> MTSTAVEITVKNAADIAIIGGSGLYQMQALTNKRSVKIETPYGEPSDDIVLGELNGVTVAFLTRHGQGHRLTPSEVPYRANIYALKTLGVRYIVSVSAVGSLQETLKPLDMVIPDQMIDMTKQRVSTFFGDGAVAHVSMADPLCPEVADILIRAYDNADIADGQCHAKATYVCIEGPQFSTRAESHWYRQMQADIIGMTNMPEAKLAREASIAYATLALVTDFDCWHPNEQAVSADYAIQNLMKNADNAQQVIKQAVALIASEQPKSIAHTALTQALVTPVEAMSAETKTRLAALLP

The monomer of RSFP has a mixed α-β architecture. The main structural motif is an eight stranded mixed β-sheet located in the centre of the monomer. On the one side of this sheet there are two long helixes, while on the opposite side there are five helixes with additional three stranded parallel β-sheets and a complicated network of loops. The native form of this protein is a trimer that is reflected in the crystal symmetry.

Analysis of the Matthews volume for the native RSFP crystal indicates the presence of one molecule in the asymmetric unit (VM = 2.37 Da·Å−3 solvent content 48.14%). The sequence identity of the investigated protein to the search models was 47%, 46% and 49% respectively. The last one had the best statistics in the Phaser program and this solution was used for further structure refinement. In the presented crystal structures the monomer is an asymmetric unit. The trimer assembly is built on a crystallographic 63-fold axis. The structures of the apo RSFP and its complex with RB are very similar; the rmsd of the superposed monomers is 0.571 Å.> GSAKDVKFGADARALMLQGVDLLADAVAVTMGPKGRTVIIEQSWGSPKVTKDGVTVAKSIDLKDKYKNIGAKLVQDVANNTNEEAGDGTTTATVLARSIAKEGFEKISKGANPVEIRRGVMLAVDAVIAELKKQSKPVTTPEEIAQVATISANGDKEIGNIISDAMKKVGRKGVITVKDGKTLNDELEIIEGMKFDRGYISPYFINTSKGQKCEFQDAYVLLSEKKISSIQSIVPALEIANAHRK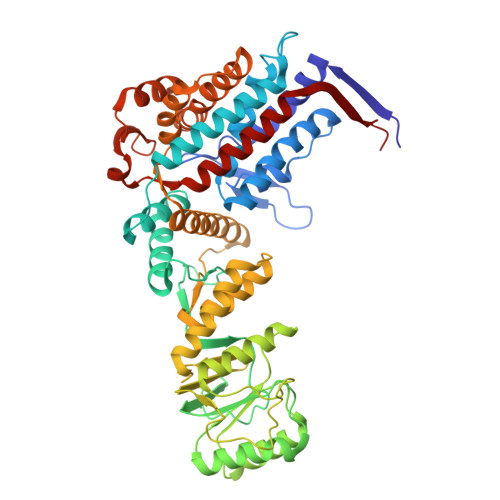PLVIIAEDVDGEALSTLVLNRLKVGLQVVAVKAPGFGDNRKNQLKDMAIATGGAVFGEEGLTLNLEDVQPHDLGKVGEVIVTKDDAMLLKGKGDKAQIEKRIQEIIEQLDVTTSEYEKEKLNERLAKLSDGVAVLKVGGTSDVEVNEKKDRVTDALNATRAAVEEGIVLGGGCALLRCIPALDSLTPANEDQKIGIEIIKRTLKIPAMTIAKNAGVEGSLIVEKIMQSSSEVGYDAMAGDFVNMVEKGIIDPTKVVRTALLDAAGVASLLTTAEVVVTEIPKE Small self‐cleaving ribozymes catalyze site‐specific cleavage of their own phosphodiester backbone. They are widely distributed in nature and are essential for rolling‐circle‐based replication of satellite and pathogenic RNAs. Comparative genomic analysis led to the discovery of novel self‐cleaving ribozymes, named twister, twister‐sister, pistol, and hatchet. In the present study we set out to obtain conformational snapshots along the reaction coordinate of the pistol ribozyme phosphordiester cleavage. We succeeded in solving the X‐ray structures of both its TS analogue vanadate (at 2.8 Å resolution) and the ternary 2′,3′ cyclophosphate product complex (at 2.65 Å resolution; see Figure S1 in the Suppporting Information for stereoviews).

To increase our understanding of the pistol ribozyme's catalytic mechanism, we have now determined its structure when complexed with a TS mimic at 2.8 Å resolution. To obtain the crystal structure of the TS analogue, we mixed the three RNA strands shown in Figure S2. The resulting complex lacks the scissile phosphate but retains the 2′‐, 3′‐, and 5′‐hydroxy groups at the cleavage site. This complex was co‐crystallized with NH4VO3. The electron density in the active site can be assigned to vanadate based on its size, shape, and anomalous scattering. As a result, the divalent metal ion (whose innersphere coordination to N7‐G33 was verified by the anomalous signal in the structure of Mn2+ soaked crystals) potentially interacts through water‐mediated hydrogen bonding with the nonbridging oxygen atoms of the scissile phosphate. This ion is also at a 4 Å distance to the 5′O leaving group of U54 such that it could position a water molecule to serve as a general acid, in the cleavage reaction, for proton transfer to stabilize the leaving 5′O. Furthermore, because the activity was not restored by addition of Mn2+ ions, water‐mediated (outersphere) rather than innersphere coordination between the phosphorothioate and the metal ion is likely and the M2+‐′proR‐O′ distance of 3.3 Å in our TS structure supports this notion further. In the TS, the nucleobase of G40 stabilizes the phosphorane in a bidendate manner (via N1⋅⋅⋅2′O and N2⋅⋅⋅pro‐R O), and simultaneously, the proximity of the divalent ion that remains innersphere‐coordinated to N7 of G33 assists in lowering the energy barrier by electrostatic interactions and by outershell coordination to the pro‐R nonbridging oxygen atom of the scissile phosphate. This process, in turn, places one of its first shell water molecules into appropriate distance for proton transfer (general acid) to the 5′O leaving group.

>[2x]ACUCGUUUGAGCGAGUAUAAACAGUUGGUUAGGCUCAAAGCGGAGAGCAG;>UCUGCUCUCXUCCAA[2x]>MVPKVYAGQEMAMVENENCIMNGKWKKRVHVFGERVMRFPNKAWQTTWKVGREDPRRLIHAFKVGLSLTLASLLYLLEPLFKGIGQSAIWAVMTVVVVLEFTAGATLCKGLNRGLGTLLAGLLAFLVGYIANASDRVSQAIIIGAAVFFIGALATYMRFIPYIKKNYDYGLVIFLLTFNLITVSSYRLENVLKIAHDRVYTIAIGCAVCLLMSLLVFPNWSGEDLHNSTVYKLEGLAKSIEACVNEYFYGEIEGSGYMKLSEDPIYKGYKAVLDSKSIDETLALHASWEPRHSRYCHRFPWQQYVKVGAVLRQFGYTVVALHGCLRTEIQTP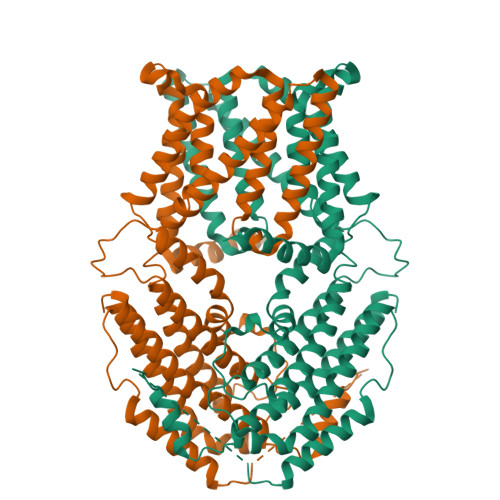RSVRAMFKDPCIRLAAEVSKVLIELSNSIRNRRHCSPEILSDHLHEALQDLNTAIKSQPRLFLGPKHRHNQATNMLKIAAAQVGQERHGKTSLSSVKTDSSALLEWKTKRVSAEQTKESERKSLRPQLSKIAITSLEFSEALPFAAFASLLVETVAKLDLVIEEVEELGRLACFKEFIPGDEFVVTCQEPRVDVSQNHLPSHGVD[2x]>MTSTGRFTLPSEENFAEKTKELAELWGADAIRNSDGTHLDEAVLALGKKIYNAYFPTRAHNEWITLHMDETPQVYLLTDRILAESDTVDIPLMESFFAEQLKPNRDADPHKYWEVVDRTTGEVVDSANWTLDADEDTVHVSGVAAWHEYTVSFLAYIIWDPVEMYNHLTNDWGDKEHEIPFDIYHPATRKFVFDTFEQWLKDSPQTDVVRFTTFFYQFTLLFDEKRREKVVDWFGYACTVSPRALDDFEAKYGYRLRPEDFVDGGAYNSAWRVPRKAQRDWIDFLSGFVRENVKQLADMSHAAGKEAMMFLGDQWIGTEPYKDGFDELGLDAVVGSIGDGTTTRMIADIPGVKYTEGRFLPYFFPDTFYEGNDPSIEGLDNWRKARRAILRSPISRMGYGGYLSLAAKFPKFVDTVTHIANEFRDIHDRTGGVAAEGELNVAILNSWGKMRSWMAFTVAHALPNKQTYSYYGILESLSGMRVNVRFISFDDVLAHGIDSDIDVIINGGPVDTAFTGGDVWTNPKLVETVR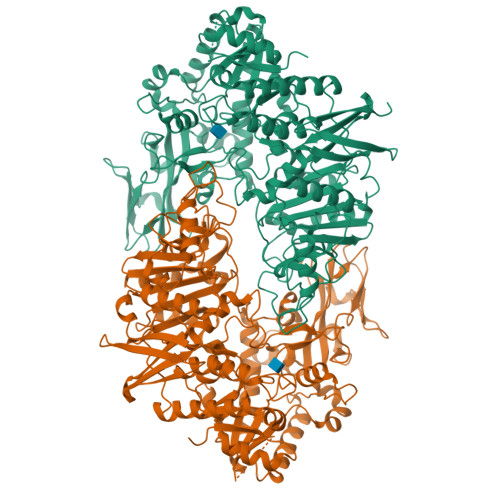AWVRGGGAFVGVGEPSSAPRFQTGRFFQLADVIGVDEERYQTLSVDKYFPPVVPDHFITADVPVDPAAREAWEQAGYRIPLSGCGGGQSIKPLGGIDFGEPVLNTYPVNENVTLLRADGGQVQLATNDYGKGRGVYISGLPYSAANARLLERVLFYASHNEDKYAAWSSSNPECEVAHFPEQGLYCVINNTDQPQKTTVTLADGTTEDFDLPDSGIAWREALEHHHHHH[4x]> MATDVA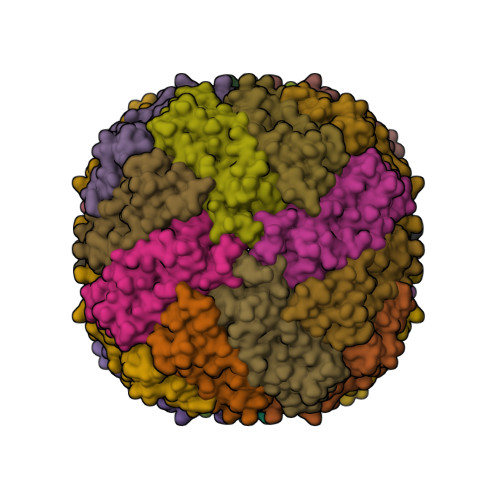QGPNGRALAESMNPDLLSAIQQHISIERYASVTFLAMSIWCAERELAGFYQFFDGEAKDEQSHAVHFTQYLIARSQSNDLQTLDAPRQNWDSLASLMATAFQMEADTTSSIQSVYALAERNSDTRTTVFLDPLIEAQIQSEDQFAYLLGRVKFANGDPTALLVIDNELRAGQTQRG4-HYDROXY-1,2,5-THIADIAZOLE-3-CARBOXYLIC 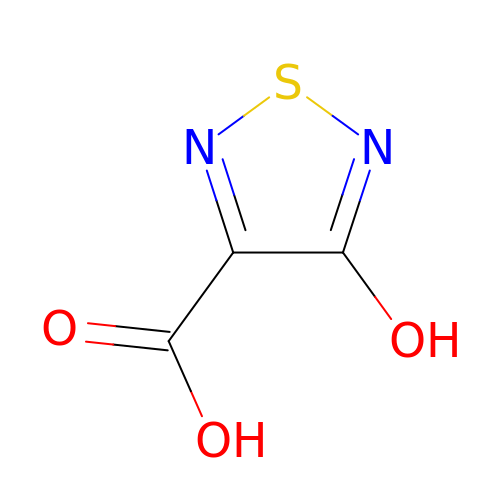ACID | C3 H2 N2 O3 S | FVZITYNLUYJDOE-UHFFFAOYSA-N> MGMWASLDALWEMPAEKRIFGAVLLFSWTVYLWETFLAQRQRRIYKTTTHVPPELGQIMDSETFEKSRLYQLDKSTFSFWSGLYSETEGTLILLFGGIPYLWRLSGRFCGYAGFGPEYEITQSLVFLLLATLFSALTGLPWSLYNTFVIEEKHGFNQQTLGFFMKDAIKKFVVTQCILLPVSSLLLYIIKIGGDYFFIYAWLFTLVVSLVLVTIYADYIAPLFDKFTPLPEGKLKEEIEVMAKSIDFPLTKVYVVEGSKRSSHSNAYFYGFFKNKRIVLFDTLLEEYSVLNKDIQEDSGMEPRNEEEGNSEEIKAKVKNKKQGCKNEEVLAVLGHELGHWKLGHTVKNIIISQMNSFLCFFLFAVLIGRKELFAAFGFYDSQPTLIGLLIIFQFIFSPYNEVLSFCLTVLSRRFEFQADAFAKKLGKAK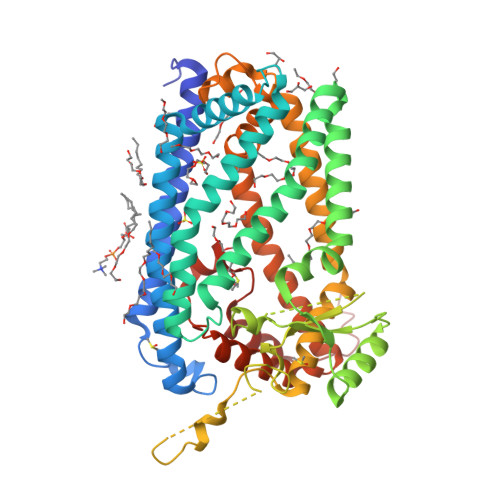DLYSALIKLNKDNLGFPVSDWLFSMWHYSHPPLLERLQALKTMKQSGLEVL> MSSITSETGKRRVKRTYEVTRQNDNAVRIEPSSLGEEEDKEAKDKNSALQLKRSRYDPNKVFSNTNQGPEKNNLKGEQLGSQKKSSKYDEKITSNNELTTKKGLLGDS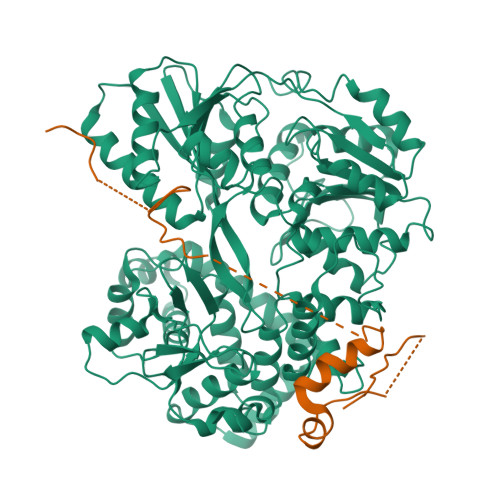ENETKYASSNSKFNVEVTHKIKNAKEIDKINRQRMWEEQQLRNAMAGQSDHPDDITLEGSDKYDYVFDTDAMIDYTNEEDDLLPEEKLQYEARLAQALETEEKRILTIQEARKLLPVHQYKDELLQEIKKNQVLIIMGETGSGKTTQLPQYLVEDGFTDQGKLQIAITQPRRVAATSVAARVADEMNVVLGKEVGYQIRFEDKTTPNKTVLKYMTDGMLLREFLTDSKLSKYSCIMIDEAHERTLATDILIGLLKDILPQRPTLKLLISSATMNAKKFSEFFDNCPIFNVPGRRYPVDIHYTLQPEANYIHAAITTIFQIHTTQSLPGDILVFLTGQEEIERTKTKLEEIMSKLGSRTKQMIITPIYANLPQEQQLKIFQPTPENCRKVVLATNIAETSLTIDGIRYVIDPGFVKENSYVPSTGMTQLLTVPCSRASVDQRAGRAGRVGPGKCFRIFTKWSYLHELELMPKPEITRTNLSNTVLLLLSLGVTDLIKFPLMDKPSIPTLRKSLENLYILGALNSKGTITRLGKMMCEFPCEPEFAKVLYTAATHEQCQGVLEECLTIVSMLHETPSLFIGQKRDAAASVLSEVESDHILYLEIFNQWRNSKFSRSWCQDHKIQFKTMLRVRNIRNQLFRCSEKVGLVEKNDQARMKIGNIAGYINARITRCFISGFPMNIVQLGPTGYQTMGRSSGGLNVSVHPTSILFVNHKEKAQRPSKYVLYQQLMLTSKEFIRDCLVIPKEEWLIDMVPQIFKDLIDDKTNRGRR;> MSKFSLKLGSKTLKKNISKKTKKKNSLQKANLFDWDDAETASLSHKPQSKIKIQSIDKFDLDEESSSKKKLVIKLSENADTKKNDAPLVEYVTEKEYNEVPVEEFGDALLRGMGWESDSEQDSKGDKTQSRNKDVSNVSQIHPDGLGIGAKLNKAINVEEASFMPVVKIDKITGTKVDDDKKNKS RESORCINOL | C6 H6 O2 | 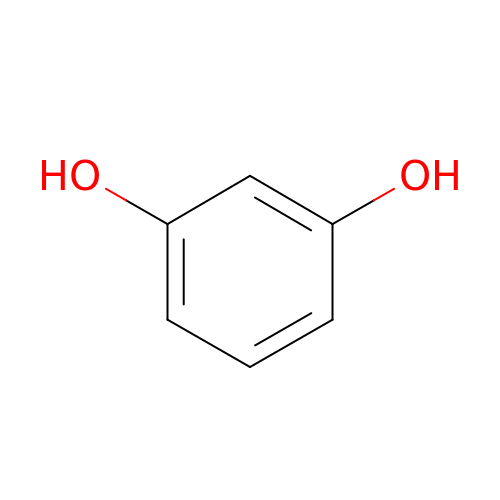GHMLBKRAJCXXBS-UHFFFAOYSA-N>[3x]VPQNPNVLVWMDLEMTGLDPEKDRIIEMATIITDGDLRTIAEGPVIVIHQKQELIDGMDEWNTRTHNK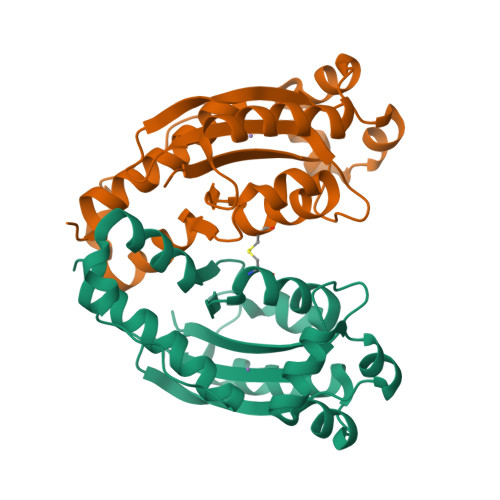TGLVTKVKTSRVTERQAEIETLDFIQRHTLKNRAPLCGNSICQDRRFLYKYMPELSEWLHYRNVDVSSFKEVARHWAPSILSGFEKRASHQALDDIKESIEELRYYRNNLILLDMN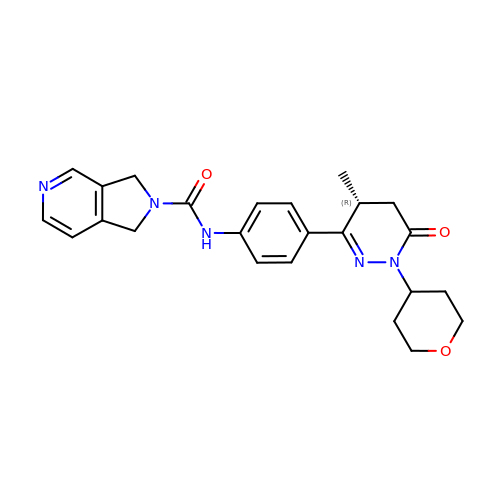N-[4-[(4R)-4-methyl-1-(oxan-4-yl)-6-oxidanylidene-4,5-dihydropyridazin-3-yl]phenyl]-1,3-dihydropyrrolo[3,4-c]pyridine-2-carboxamide | C24 H27 N5 O3 | YFHOMYWNYOHHDS-MRXNPFEDSA-N> MANVPWAEVCEKFQAALALSRVELHKNPEKEPYKSKYSARALLEEVKALLGPAPEDEDERPEAEDGPGAGDHALGLPAEVVEPEGPVAQRAVRLAVIEFHLGVNHIDTEELSAGEEHLVKCLRLLRRYRLSHDCISLCIQAQNNLGILWSEREEIETAQAYLESSEALYNQYMKEVGSPPLDPTERFLPEEEKLTEQERSKRFEKVYTHNLYYLAQVYQH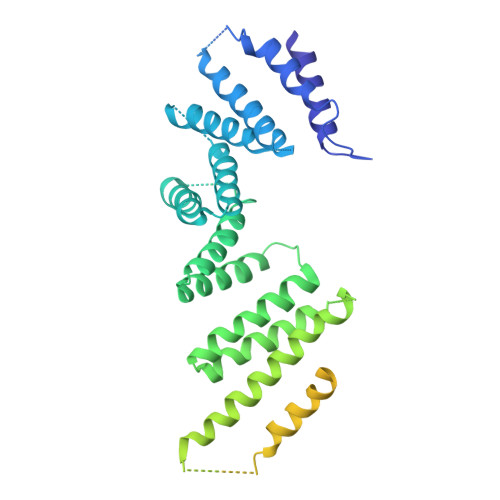LEMFEKAAHYCHSTLKRQLEHNAYHPIEWAINAATLSQFYINKLCFMEARHCLSAANVIFGQTGKISATEDTPEAEGEVPELYHQRKGEIARCWIKYCLTLMQNAQLSMQDNIGELDLDKQSELRALRKKELDEEESIRKKAVQFGTGELCDAISAVEEKVSYLRPLDFEEARELFLLGQHYVFEAKEFFQIDGYVTDHIEVVQDHSALFKVLAFFETDMERRCKMHKRRIAMLEPLTVDLNPQYYLLVNRQIQFEIAHAYYDMMDLKVAIADRLRDPDSHIVKKINNLNKSALKYYQLFLDSLRDPNKVFPEHIGEDVLRPAMLAKFRVARLYGKIITADPKKELENLATSLEHYKFIVDYCEKHPEAAQEIEVELELSKEMVSLLPTKMERFRTKMALT> LVV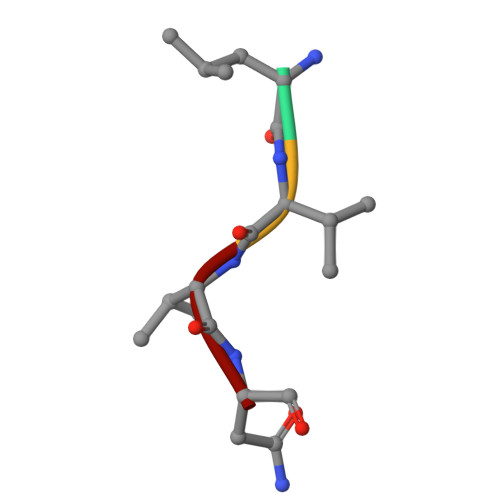N>MDFPRIIMARNPIYFESIQIGEKIEGLPRTVTETDIWTFAYLTADFFPLHTDVEFAKKTIFGKPIAQGMLVLSIALGMVDQVILSNYDVSSVIAFFGIKDVRFLRPVFIGDTIAASAEVVEKQDFDEKSGVVTYKLEVKNQRGELVL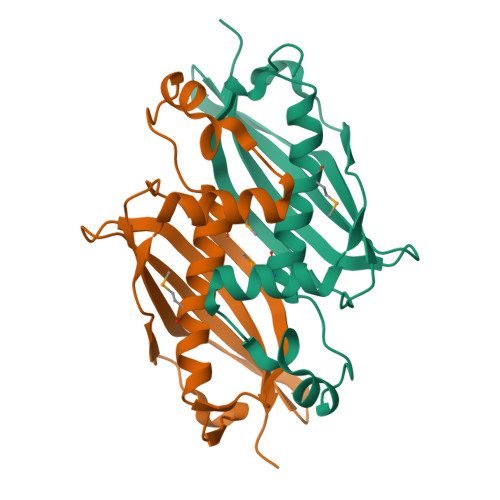TALYSALIRKTPSK[12x]> PLREGRGL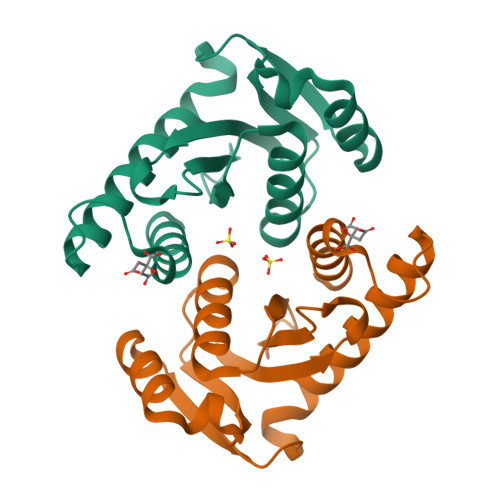GPLQIWQTNFTLEPRMAPRSWLAVTVDTASSAIVVTQHGRVTSVAAQHHWATAIAVLGRPKAIKTDNGSCFTSKSTREWLARWGIAHTTGIPGNSQGQAMVERANRLLKDKIRVLAEGDGFMKRIPTSKQGELLAKAMYALNHFERGENTKTNL(4aS,8aR)-4a,5,6,7,8,8a-hexahydro-4H-3,1-benzothiazin-2-amine | 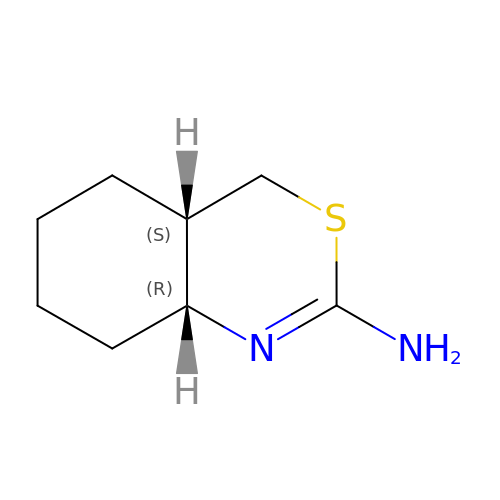C8 H14 N2 S | SZAFVQHJBWFBIQ-RNFRBKRXSA-N> ALWQFNGMIKCKIPSSEPLLDFNNYGCYCGLGGSGTPVDDLDRCCQTHDNCYMQAMKLDSCKVLVDNPYTNNYSYSCSNNEITCSSENNACEAFICNCDRNAAICFSKVPYNKEHKNLDK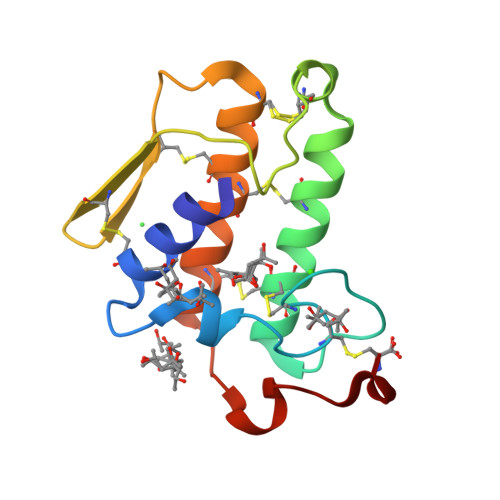KNC>GIDPFTDREKQQLSIEAARLYYQSDYSQQQIAEQLNISRPTVSRLLQYAKEKGYVQIRVMDPFEDLDALGSILEEKYGLLEAHVVFSPTPDYAGITHDLSRYGAEYMHETVKDGDIVGVSWGTTMYQIAQNMQPKQVKGVEVVQLKGGISHSRVNTYSAETIQLFAEAFQTMPRYLPLPVVFDNADVKRMVEKDRHIERIIEMGKQANIALFTVGTVRDEALLFRLGYFNEEEKALLKKQAVGDICSRFFDAKGNICSSAINDRTIGVELQDLRLKERSILVAGGSRKVSSIHGALTGKYANVLIIDQHTARALVNDL[4x]

The SorC family of transcriptional regulators plays a crucial role in controlling the carbohydrate metabolism and quorum sensing. A typical SorC protein comprises an N-terminal DNA-binding domain (DBD) of a helix–turn–helix (HTH) motif, along with a C-terminal Rossmann-like fold effector-binding domain (EBD). SorC repressors generally form tetramers as they bind to their operators located in promoter regions of regulated genes.

DeoR acts as a repressor of the dra–nupC–pdp operon, which encodes catabolic enzymes for the utilization of deoxyribose and deoxyribonucleoside when other preferred carbon sources are lacking. Successful crystallization was achieved for a complex with an 18 bp long DNA duplex (referred to here as OL18) that contained the first two palindromic binding sites of the operator (5′-ATTGAACAAAATTTCAAT-3′), specifically the left-half operator sequence. The crystal structure was determined by molecular replacement and refined to a resolution of 3.7 Å. The asymmetric unit comprised two physiological protein dimers, each bound to one OL18 duplex. Each monomer within the dimer contains an N-terminal HTH-type domain and a C-terminal effector-binding domain of a three-layer (α/β/α) sandwich architecture containing a double Rossmann fold. The antiparallel β-sheet formed upon DBD dimerization results in swapped positions of the EBD domains with respect to the N-terminal DBDs. The dimeric interface is provided only by the N-terminal domains; interactions of the C-terminal domains within the dimer are negligible. Within the crystal, this interaction was observed between two symmetry-related DeoR dimers originating from the neighboring asymmetric unit. The DeoR dimer interacts with the major DNA groove and the DBDs within each dimer are spatially separated by about one DNA turn. A tetrameric assembly is formed through the interaction of EBDs with the dimer from the neighboring asymmetric unit in the crystal lattice, and this crystallographic tetramer allowed us to construct our biologically relevant model of DeoR bound to the full operator.>[4x]GSSGSSGMDPNTVSSFQVDCFLWHVRKRLADQELGDAPF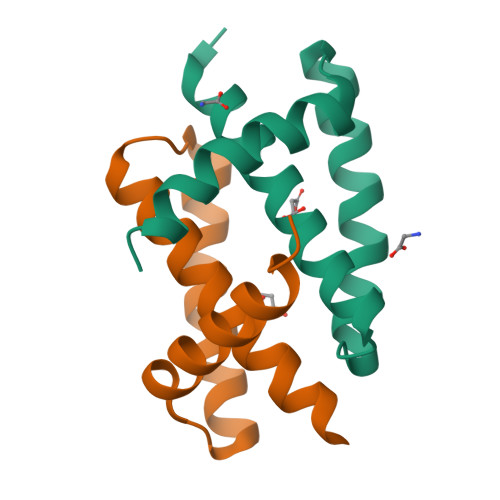LDRLRRDQKSLRGRGNTLGLDIETATRAGKQIVERILEEE>[2x]MTTQVKHFETLMPGYDSWIYIDLETGKFEQQAE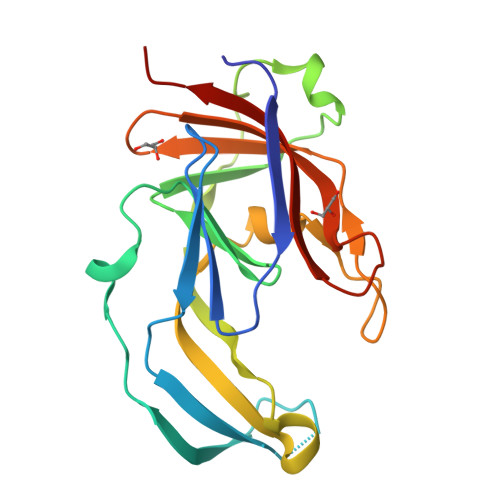LGKREFRKYKSMMDPNYEVVGTEPAKGTDADLPKKWDIAFHITDARTNNGEVLMTGETDLNKINALPAGNYVADAPADIVVDMSRMQSEGVLGMVKTMLNGEMGKWVKSNGMGKPKTVMGNVFAVKFKNGNAALIKFKDNLDKTGKKKAVSFDYKFIKKAK>GVFVFRDE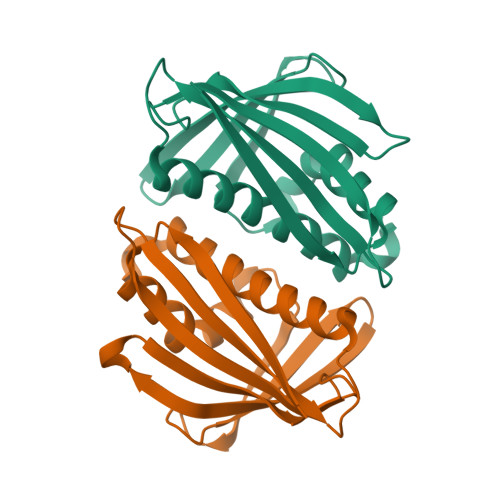TSSSVAPAKLYKALTKDSDTIAQKIDGPIQSIELVEGNGGVGTIKKITANEGDKTSFVLQKVDAIDEANLGYDYSIVGGTGLPESLEKLSFETKVVAGSGGGSISKVTLKFHTKGDAPLSDAVRDDALAKGAGFFKAIEGYVLANPAEY[2x]> MEEGARHRNNTEKKHPGGGESDASPEAGSGGGGVALKKEIGLVSACGIIVGNIIGSGIFVSPKGVLENAGSVGLALIVWIVTGFITVVGALCYAELGVTIPKSGGDYSYVKDIFGGLAGFLRLWIAVLVIYPTNQAVIALTFSNYVLQPLFPTCFPPESGLRLLAAICLLLLTWVNCSSVRWATRVQDIFTAGKLLALALIIIMGIVQICKGEYFWLEPKNAFENFQEPDIGLVALAFLQGSFAYGGWNFLNYVTEELVDPYKNLPRAIFISIPLVTFVYVFANVAYVTAMSPQELLASNAVAVTFGEKLLGVMA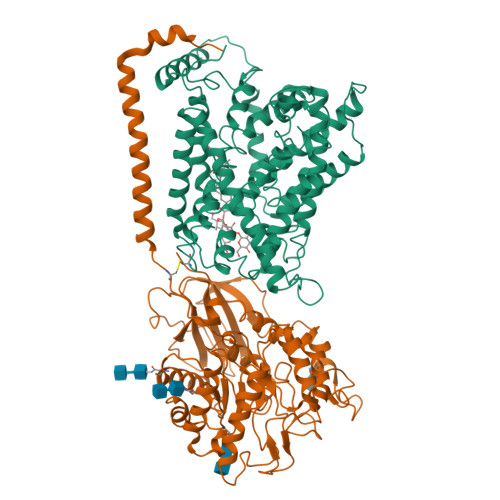WIMPISVALSTFGGVNGSLFTSSRLFFAGAREGHLPSVLAMIHVKRCTPIPALLFTCISTLLMLVTSDMYTLINYVGFINYLFYGVTVAGQIVLRWKKPDIPRPIKINLLFPIIYLLFWAFLLVFSLWSEPVVCGIGLAIMLTGVPVYFLGVYWQHKPKCFSDFIELLTLVSQKMCVVVYPEVERGSGTEEANEDMEEQQQPMYQPTPTKDKDVAGQPQP;> MSQDTEVDMKEVELNELEPEKQPMNAASGAAMSLAGAEKNGLVKIKVAEDEAEAAAAAKFTGLSKEELLKVAGSPGWVRTRWALLLLFWLGWLGMLAGAVVIIVRAPRCRELPAQKWWHTGALYRIGDLQAFQGHGAGNLAGLKGRLDYLSSLKVKGLVLGPIHKNQKDDVAQTDLLQIDPNFGSKEDFDSLLQSAKKKSIRVILDLTPNYRGENSWFSTQVDTVATKVKDALEFWLQAGVDGFQVRDIENLKDASSFLAEWQNITKGFSEDRLLIAGTNSSDLQQILSLLESNKDLLLTSSYLSDSGSTGEHTKSLVTQYLNATGNRWCSWSLSQARLLTSFLPAQLLRLYQLMLFTLPGTPVFSYGDEIGLDAAALPGQPMEAPVMLWDESSFPDIPGAVSANMTVKGQSEDPGSLLSLFRRLSDQRSKERSLLHGDFHAFSAGPGLFSYIRHWDQNERFLVVLNFGDVGLSAGLQASDLPASASLPAKADLLLSTQPGREEGSPLELERLKLEPHEGLLLRFPYAA>SEEPPFDIRALRADIEDMISEKLELGPSLIRL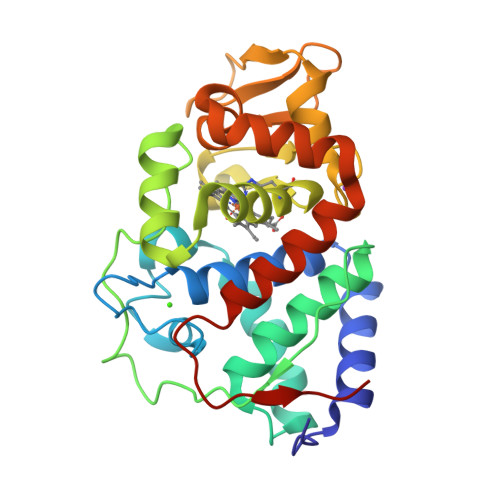AWHEAASYDCFKKDGSPNSASMRFKPECLYAGNKGLDIPRKALETLKKKYPQISYADLWVLAAYVAIEYMGGPTIPFCWGRVDAKDGSVCGPDGRLPDGSKTQSHVREVFRRLGFNDQETVALIGAHTCGECHIEFSGYHGPWTHRKNGFDNSFFTQLLDEDWVLNPKVEQMQLMDRATTKLMMLPSDVCLLLDPSYRKYVELYAKDNDRFNKDFANAFKKLTELGTRNLHKAPASES[2x]>[2x]AMKDHKFWRTQPVKDFDEKVVEEGPIDKPKTPEDISDKPLPLLSSFEWCSIDVDNKKQLEDVFVLLNENYVEDRDAGFRFNYTKEFFNWALKSPGWKKDWHIGVRVKETQKLVAFISAIPVTLGVRGKQVPSVEINFLCVHKQLRSKRLTPVLIKEITRRVNKCDIWHALYTAGIVLPAPVSTCRYTHRPLNWKKLYEVDFTGLPDGHTEEDMIAENALPAKTKTAGLRKLKKEDIDQVFELFKRYQSR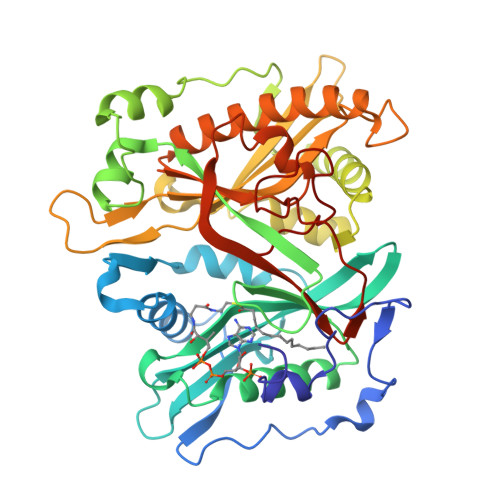FELIQIFTKEEFEHNFIGEESLPLDKQVIFSYVVEQPDGKITDFFSFYSLPFTILNNTKYKDLGIGYLYYYATDADFQFKDRFDPKATKALKTRLCELIYDACILAKNANMDVFNALTSQDNTLFLDDLKFGPGDGFLNFYLFNYRAKPITGGLNPDNSNDIKRRSNVGVVML>MADLSSRVNELHDLLNQYSYEYYVEDNPSVPDSEYDKLLHELIKIEEEHPEYKTVDSPTVRVGGEAQASFNKVNHDTPMLSLGNAFNEDDLRKFDQRIREQIGNVEYMCELKIDGLAVSLKYVDGYFVQGLTRGDGTTGEDITENLKTIHAIPLKMKEPLNVEVRGEAYMPRRSFLRLNEEKEKNDEQLFANPRNAAAGSLRQLDSKLTAKRKLSVFIYSVNDFTDFNARSQSEALDELDKLGFTTNKNRARVNNIDGVLEYIEKWTSQRESLPYDIDGIVIKVNDLDQQDEMGFTQKSPRWAIAYKFPAEEHH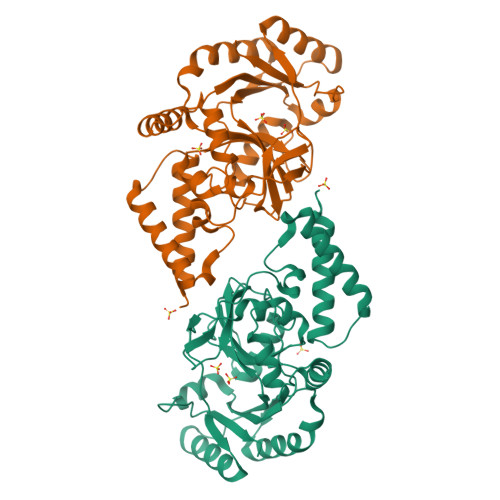HHHH[2x]> MASSRCPAPRGCRCLPGASLAWLGTVLLLLADWVLLRTALPRIFSLLVPTALPLLRVWAVGLSRWAVLWLGACGVLRATVGSKSENAGAQGWLAALKPLAAALGLALPGLALFRELISWGAPGSADSTRLLHWGSHPTAFVVSYAAALPAAALWHKLGSLWVPGGQGGSGNPVRRLLGCLGSETRRLSLFLVLVVLSSLGEMAIPFFTGRLTDWILQDGSADTFTRNLTLMSILTIASAVLEFVGDGIYNNTMGHVHSHLQGEVFGAVLRQETEFFQQNQTGNIMSRVTEDTSTLSDSLSENLSLFLWYLVRGLCLLGIMLWGSVSLTMVTLITLPLLFLLPKKVGKWYQLLEVQVRESLAKSSQVAIEALSAMPTVRSFANEEGEAQKFREKLQEIKTLNQKEAVAYAVNSWTTSISGMLLKVGILYIGGQLVTSGAVSSGNLVTFVLYQMQFTQAVEVLLSIYPRVQKAVGSSEKIFEYLDRTPRCPPSGLLTPLHLEGLVQFQDVSFAYPNRPDVLVLQGLTFTLRPGEVTALVGPNGSGKSTVAALLQNLYQPTGGQLLLDGKPLPQYEHRYLHRQVAAVGQEPQVFGRSLQENIAYGLTQKPTMEEITAAAVKSGAHSFISGLPQGYDTEVDEAGSQLSGGQRQAVALARALIRKPCVLILDDATSALDANSQLQVEQLLYESPERYSRSVLLITQHLSLVEQADHILFLEGGAIREGGTHQQLMEKKGCYWAMVQAPADAPE;> MRLPDLRPWTSLLLVDAALLWLLQGPLGTLLPQGLPGLWLEGTLRLGGLWGLLKLRGLLGFVGTLLLPLCLATPLTVSLRALVAGASRAPPARVASAPWSWLLVGYGAAGLSWSLWAVLSPPGAQEKEQDQVNNKVLMWRLLKLSRPDLPLLVAAFFFLVLAVLGETLIPHYSGRVIDILGGDFDPHAFASAIFFMCLFSFGSSLSAGCRGGCFTYTMSRINLRIREQLFSSLLRQDLGFFQETKTGELNSRLSSDTTLMSNWLPLNANVLLRSLVKVVGLYGFMLSISPRLTLLSLLHMPFTIAAEKVYNTRHQEVLREIQDAVARAGQVVREAVGGLQTVRSFGAEEHEVCRYKEALEQCRQLYWRRDLERALYLLVRRVLHLGVQMLMLSCGLQQMQDGELTQGSLLSFMIYQESVGSYVQTLVYIYGDMLSNVGAAEKVFSYMDRQPNLPSPGTLAPTTLQGVVKFQDVSFAYPNRPDRPVLKGLTFTLRPGEVTALVGPNGSGKSTVAALLQNLYQPTGGQVLLDEKPISQYEHCYLHSQVVSVGQEPVLFSGSVRNNIAYGLQSCEDDKVMAAAQAAHADDFIQEMEHGIYTDVGEKGSQLAAGQKQRLAIARALVRDPRVLILDEATSALDVQCEQALQDWNSRGDRTVLVIAHRLQTVQRAHQILVLQEGKLQKLAQL;> RRYQKSTEL

Peptides destined for display are first delivered into the endoplasmic reticulum (ER) by the transporter associated with antigen processing (TAP). TAP is a heteromeric ATP-binding cassette (ABC) transporter comprising two subunits, TAP1 and TAP2. Each subunit has an N-terminal transmembrane domain (TMD0) that interacts with other components of the larger peptide-loading complex, a six-transmembrane helical domain (TMD) that forms the translocation pathway, and a nucleotide-binding domain (NBD) that hydrolyzes ATP. In this study, we analyzed the structure of TAP in the presence and absence of peptides. These structures show that TAP suspends peptides across its transmembrane cavity, anchoring their termini in two distal binding pockets primarily through their backbone atoms.

The biochemical properties of the recombinant protein were assessed using the 9-mer peptide sequence RRYQKSTEL (b27), a well-characterized substrate transported by TAP and presented by HLA-B27 (25, 40). ATP hydrolysis was stimulated in a dose-dependent manner by b27, but not by N or C termini–modified b27, consistent with previous studies. To understand how TAP recognizes peptide antigens, we analyzed the structures of TAP in complex with b27 and two other 9-mer peptides, all of which have optimal lengths for binding. These three peptides, b27, ILKEPVHGV (a2), and QYDDAVYKL (c4), are natural products of the antigen processing pathway and are presented by HLA-B27, HLA-A2, and HLA-C4, respectively. In contrast, the b27-bound structure exhibits a different TMD configuration with a lateral opening. In contrast, structures obtained with the b27 (9-mer) and b27″ (7-mer) peptides have a lateral opening between the transmembrane (TM) helices that connects the translocation pathway to the membrane. Although this gap could provide access to the ER lumen for bound peptides, it is blocked by densities representing putative lipid molecules in both structures. Nevertheless, the peptides are suspended in a central cavity surrounded by TMs 2-6 from both TAP1 and TAP2 in all three structures. Despite their sequence diversity, the three 9-mer peptides are stabilized in the peptide-binding pocket by a common set of interactions involving backbone atoms on each end of the peptide. Furthermore, TAP2 L377 forms van der Waals interactions with the N terminus of all three peptides, and R373 interacts with the main chain atoms of a2 and c4 but not b27.7-HYDROXYSTAUROSPORINE | C28 H26 N4 O4 | 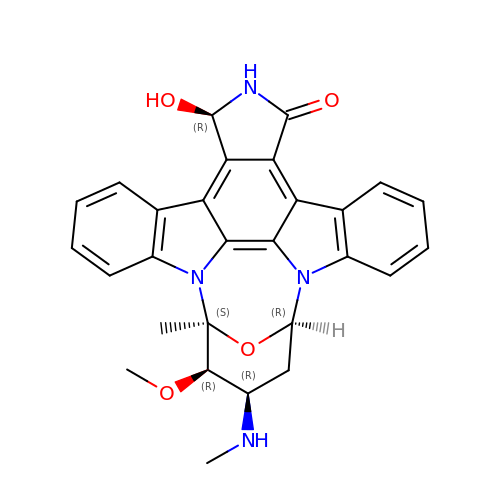PBCZSGKMGDDXIJ-HQCWYSJUSA-N> GAMGMTTYLEFIQQNEERDGVRFSWNVWPSSRLEATRMVVPVAALFTPLKERPDLPPIQYEPVLCSRTTCRAVLNPLCQVDYRAKLWACNFCYQRNQFPPSYAGISELNQPAELLPQFSSIEYVVLRGPQMPLIFLYVVDTCMEDEDLQALKESMQMSLSLLPPTALVGLITFGRMVQVHELGC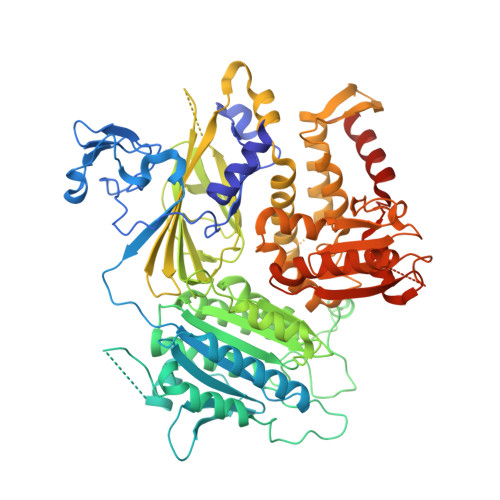EGISKSYVFRGTKDLSAKQLQEMLGLSKVPVTQATRGPQVQQPPPSNRFLQPVQKIDMNLTDLLGELQRDPWPVPQGKRPLRSSGVALSIAVGLLECTFPNTGARIMMFIGGPATQGPGMVVGDELKTPIRSWHDIDKDNAKYVKKGTKHFEALANRAATTGHVIDIYACALDQTGLLEMKCCPNLTGGYMVMGDSFNTSLFKQTFQRVFTKDMHGQFKMGFGGTLEIKTSREIKISGAIGPCVSLNSKGPCVSENEIGTGGTCQWKICGLSPTTTLAIYFEVVNQHNAPIPQGGRGAIQFVTQYQHSSGQRRIRVTTIARNWADAQTQIQNIAASFDQEAAAILMARLAIYRAETEEGPDVLRWLDRQLIRLCQKFGEYHKDDPSSFRFSETFSLYPQFMFHLRRSSFLQVFNNSPDESSYYRHHFMRQDLTQSLIMIQPILYAYSFSGPPEPVLLDSSSILADRILLMDTFFQILIYHGETIAQWRKSGYQDMPEYENFRHLLQAPVDDAQEILHSRFPMPRYIDTEHGGSQARFLLSKVNPSQTHNNMYAWGQESGAPILTDDVSLQVFMDHLKKLAVSSAA ADAMANTANE | C10 H16 | 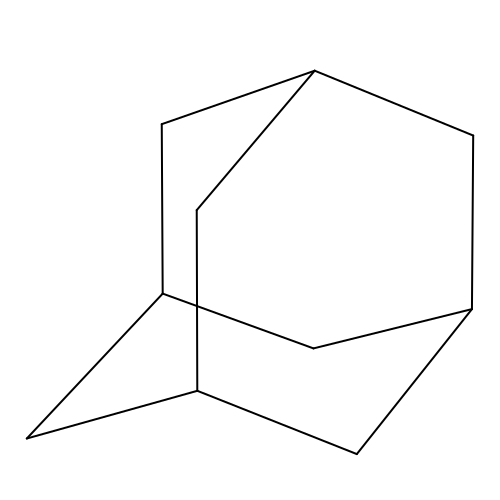ORILYTVJVMAKLC-YNFQOJQRSA-N> HHHHHHMIVLFVDFDYFYAQVEEVLNPSLKGKPVVVCVFSGRFEDSGAVATANYEARKFGVKAGIPIVEAKKILPNAVYLPMRKEVYQQVSSRIMNLLREYSEKIEIASIDEAYLDI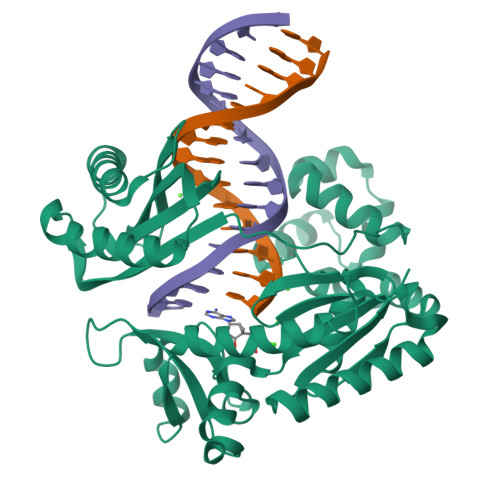SDKVRDYREAYNLGLEIKNKILEKEKITVTVGISKNKVFAKIAADMAKPNGIKVIDDEEVKRLIRELDIADVPGIGNITAEKLKKLGINKLVDTLSIEFDKLKGMIGEAKAKYLISLARDEYNEPIRTRVRKSIGRIVTMKRNSRNLEEIKPYLFRAIEESYYKLDKRIPKAIHVVAVTEDLDIVSRGRTFPHGISKETAYSESVKLLQKILEEDERKIRRIGVRFSKFIEAIGLDKFFDT> 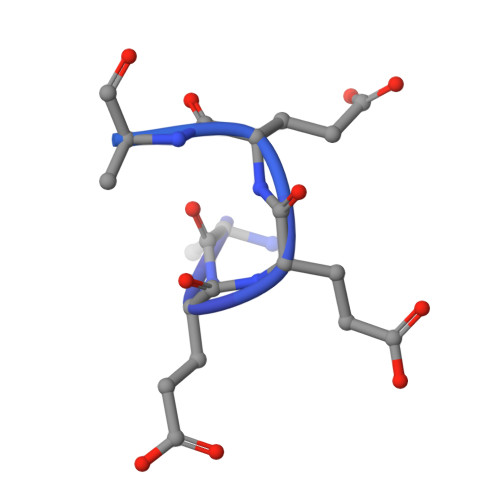EEEEEEEEEEEEEEEEEEEEEEEEEEEEEEEEEEEEEEEEEEEEEEEEEEEEEEEEEEEE>[16x]MPLKQASSNTEADERFQALLTNVNAVRAIADAVEGTLGPKGLDVMLVDKFGEVTITNDGVTILDQMDVQHPAARMLIQVARAQEEEVGDGTTTATVLAGALVSEGVNQVEQGVPVSRVIEGLRRGVERALELLRKQALPVEGLDDPRLRAVARIAAREREDIADLVVEAARHIGEDKLQDPNFKLADTVTAREGAENQVIEGVVLNKQPLNKEMPKKLEDARVLVLDDPLEPEEIDEEALSTEAGFARYLEAQEEFRENLEKLVELGVKLVLCEKGIDDTAE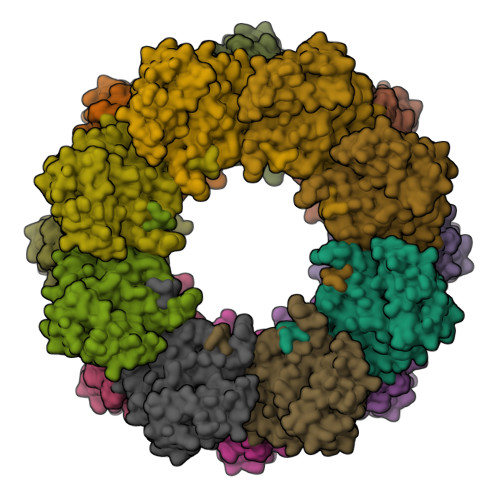ELLAEAGIMAIQRVSRKDLERVAEFTGARPVKRTALNKDAEELAKLLGHAERVRYDEKLEHVCLSGGSGEPIATVLVGAATEEVVGERERVAKDAASAVQAAIRGGVVPGGGAAELAVAREVEKLAEEVKGMERYGVEAVAEALKKPLRQIVANAGFNPLEKLGDLRAAHRTGNDSLGIDCDTGEVVDMWEAGVIDPAPVKLHALKAAGEVAAAILRINTIIKMKETGPDGGEDRG> EKPLRKLAFADLLQATNGFHNDSLIGSGGFGDVYKAILKDGSAVAIKKLIHVSGQGDREFMAEMETIGKIKHRNLVPLLGYCKVGDERLLVYEFMKYG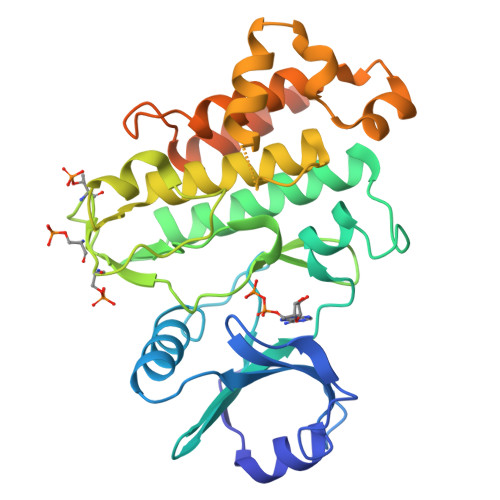SLEDVLHDPKKAGVKLNWSTRRKIAIGSARGLAFLHHNCSPHIIHRDMKSSNVLLDENLEARVSDFGMARLMSAMDTHLSVSTLAGTPGYVPPEYYQSFRCSTKGDVYSYGVVLLELLTGKRPTDSPDFGDNNLVGWVKQHAKLRISDVFDPELMKEDPALEIELLQHLKVAVACLDDRAWRRPTMVQVMAMFKEIQAGSGIDSQSTIRSIEDGGFSTIEMVDMSIKEVPEGKL>[2x]SDSFWEPGNYKRTTKRIEDGYKLCNDLQQLIQE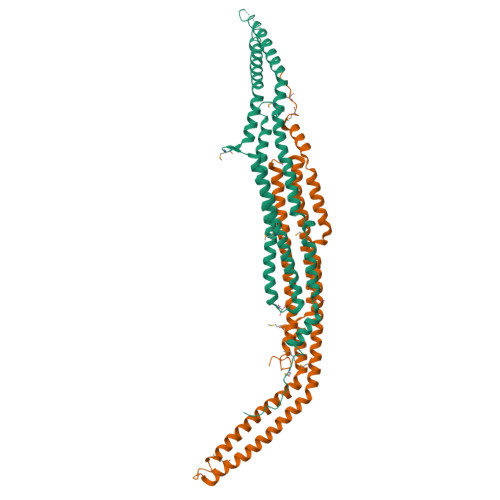RADIEKGYAKSLRTWSKKWGELIEKGPEYGTTEAAWKGVLTESERISDVHMKIKDNLCNDVNSQIKTWQKENYHHTLMQIKERKDLEDLFKKAQKPWAKLLAKVEKAKADYHSACKTERSATNQERNANADSSLSPDQVKKMHDRVQKTKDQVQKCREKYEQAIAEITKYNSVYIEDMTSVFEKCQTFEKTRLQFFKEILFNVHSCLDLTKVQSLPQIYEEFSHTINNADQQKDLKWWSNNHGINMAMNWPSFVEYT>TTSSDQKCIEKEVNKTYNCENLGLNEIPGTLPNSTECLEFSFNVLPTIQNTTFSRLINLTFLDLTRCQIYWIHEDTFQSQHRLDTLVLTANPLIFMAETALSGPKALKHLFFIQTGISSIDFIPLHNQKTLESLYLGSNHISSIKLPKGFPTEKLKVLDFQNNAIHYLSKEDMSSLQQATNLSLNLNGNDIAGIEPGAFDSAVFQSLNFGGTQNLLVIFKGLKNSTIQSLWLGTFEDMDDEDISPAVFEGLCEMSVESINLQKHYFFNISSNTFHCFSGLQELDLTATHLSELPSGLVGLSTLKKLVLSANKFENLCQISASNFPSLTHLSIKGNTKRLELGTGCLENLENLRELDLSHDDIETSDCCNLQLRNLSHLQSLNLSYNEPLSLKTEAFKECPQLELLDLAFTRLKVKDAQSPFQNLHLLKVLNLSHSLLDISSEQLFDGLPALQHLNLQGNHFPKGNIQKTNSLQTLGRLEILVLSFCDLSSIDQHAFTSLKMMNHVDLSHNRLTSSSIEALSHLKGIYLNLASNHISIILPSLLPILSQQRTINLRQNPLDCTCSNIYFLEWYKENMQKLEDTEDTLCENPPLLRGVRLSDVTLSCS[2x];>DHGSENGWPKHTACNSGGLEVVYQSCDPLQDFGLSIDQCSKQIQSNLNIRFGIILRQDIRKLFLDITLMAKGSSILNYSYPLCEEDQPKFSFCGRRKGEQIYYAGPVN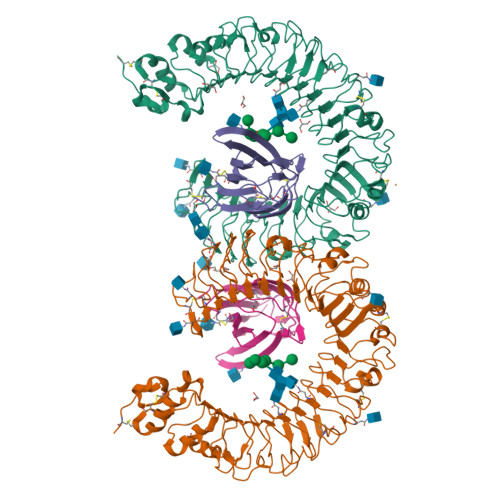NPGLDVPQGEYQLLLELYNENRATVACANATVTSSEF[2x]> AETYEGDWVDGKMQGRGTYFFADGGIYEGDWVDGKMEGKGVYKYLNGNKYEGEWINDMKNGYGTLAYVNGELYEGYWKNDKVHGKGTLTYSKGDKYIGEWKYAKKCGEGELIYASGDKFKGQWKNDKANGYGILLYNNGNKYEGEWLDDHRHGMGTFTCKEDGTIYSGHFQFNRKHGKGTLTFVNGHILQGIWNSGLLEKVINYELTPSSPWNDPDL

High-resolution crystal structures and biophysical analyses of a truncated form of the TbMORN1 protein and its homologues from the parasites Toxoplasma gondii (TgMORN1) and Plasmodium falciparum (PfMORN1) enabled, for the first time, a structure-based definition of the MORN repeat. All three structures are antiparallel dimers joined via their C-termini, and, when possessed of the correct key residues, can adopt extended or V-shaped quaternary structures. The crystal structures confirmed that each 23-amino acid MORN repeat is composed of a β-hairpin followed by a 6-residue loop that connects to the next MORN repeat. The structural studies presented here make a case that one conserved function of MORN repeats is in homotypic interactions and possibly also in higher-order assembly.

Diffracting crystals of selenomethionine-labelled PfMORN1(7–15) were obtained and its crystal structure was determined to 2.14 Å resolution using the single-wavelength anomalous dispersion (SAD) method. TbMORN1(7–15) P21, C2 and TgMORN1(7–15) crystallised with one dimer in the asymmetric unit, while PfMORN1(7–15) crystallised with one subunit in the asymmetric unit and the functional dimer was formed via crystallographic symmetry axis. Interestingly, PfMORN1(7–15) displays a V-shaped dimer with an inter-subunit angle of about 45°, and incorporates a structural Zn2+ ion at the dimer interface. Unlike the extended dimers of TbMORN1(7–15) and TgMORN1(7–15), the V-shaped PfMORN1(7–15) is mainly stabilised by a single Zn2+ ion incorporated into the core of its dimer interface, spanning over 665 Å2. The Cys306 and Asp309 residues from each subunit tetrahedrally coordinate the Zn2+ at expected distances (2.32 Å for Zn2+-S and 1.94 Å for Zn2+-O). In addition, residues from repeats 13–15 are involved in stabilising the dimer via a combination of hydrophobic, polar, and electrostatic interactions across the subunits. Although Asp residues 303 (TbMORN1), 308 (TgMORN1), and 309 (PfMORN1) are conserved in all the three proteins, the coordination of a Zn2+ ion clearly demands the presence of both cysteine and aspartate residues. Such pairs are present in PfMORN1 and TgMORN1, but not in TbMORN1, where the cysteine residue at the corresponding position is replaced by Leu301. The SAXS analysis of PfMORN1(7–15) indicated an extended structure in solution however, similar to that seen for TbMORN1(7–15) and TgMORN1(7–15) and different from the V-shaped form observed in the crystal lattice. This supports the prediction that TgMORN1 and PfMORN1 are capable of adopting two different conformations.> MSKARRWVIIVLSLAVLVMIGINMAEKDDTAQVVVNNNDPTYKSEHTDTLVYNPEGALSYRLIAQHVEYYSDQAVSWFTQPVLTTFDKDKIPTWSVKADKAKLTNDRMLYLYGHVEVNALV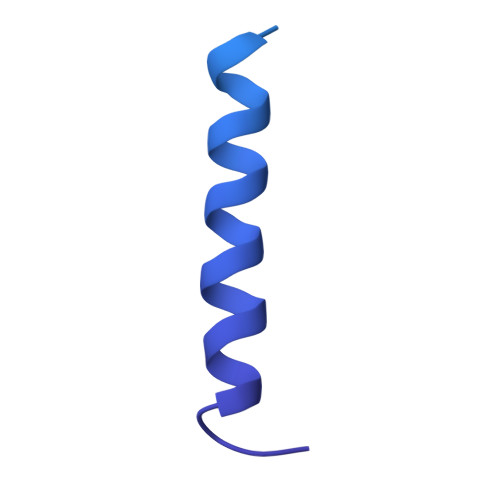PDSQLRRITTDNAQINLVTQDVTSEDLVTLYGTTFNSSGLKMRGNLRSKNAELIEKVRTSYEIQNKQTQP(E)-O-(carbamoylamino)-N-({3-hydroxy-2-methyl-5-[(phosphonooxy)methyl]pyridin-4-yl}methylidene)-L-serine 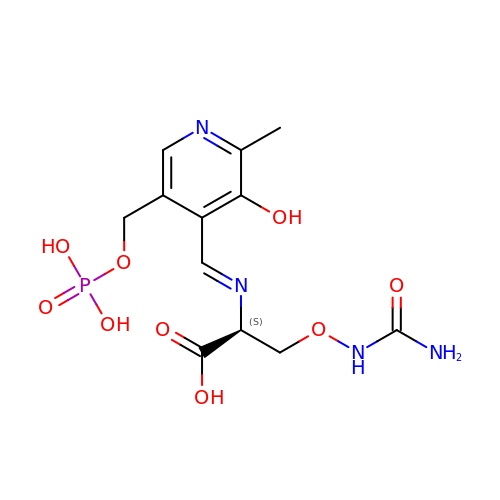| C12 H17 N4 O9 P | LKTMSPZJJUSLRR-FUOCOAHQSA-N>[4x]MIQTVEFNEQFSKALDLMENTNKNVLIVGRAGTGKSTLLNYFRNNTKKKIAVLAPTGVAAVNIKGQTIHSFFNFKPDITLSSVKDIKPKNKEIYKKLDAIVIDEVSMVRADLFDCINEFLKIHGKQPGEPFGGIQLILIGDLYQLPPVVTSSEKKFFSQIYKSPFFFDSISFNEAEFEFVELEKVYRQKDEKFIKLLNAIRNKTIEEKDLEELNKRYIPDFEPDEKEFYIYLTTTNELADKINQQKLEKLKGKKYVYQGYIEGDFSEKDLPAPLELVIKKGTQVMLLNNDYQGRWINGSMGRVVDIEKVKGNEDIIWVELEDGEEVPVQPYEWDMFEFYYDKAQKKIKSRTVGSYYQYPLKPAWAITIHKSQGLTFDKVIIDIGRGTFSHGQLYVALSRCRSLEGLVLKKPISEKYIWLDKRVVSFLTKYQYKLSSKKLPLEEKIEIIKKAISEKKPIEIVYLKSKDVKSKRVIIPKKIGKMDYNGAEFLGVEG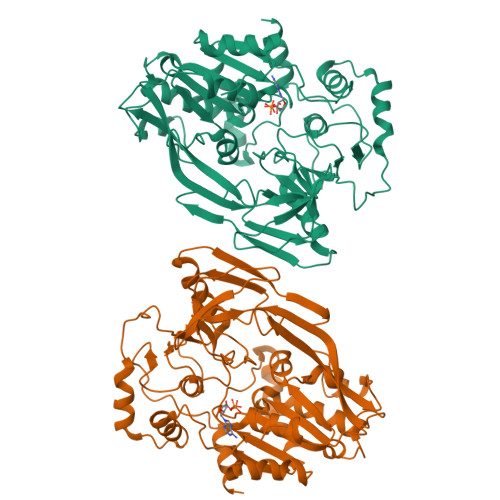FCTIRKDDRVFNVEKILEIKEIE>[2x]GSTKPFGVNRGLDLDKILHCYQMNDDLFMFVTWKGCSSIDAVHINDIKEAYPLQIIKYFESL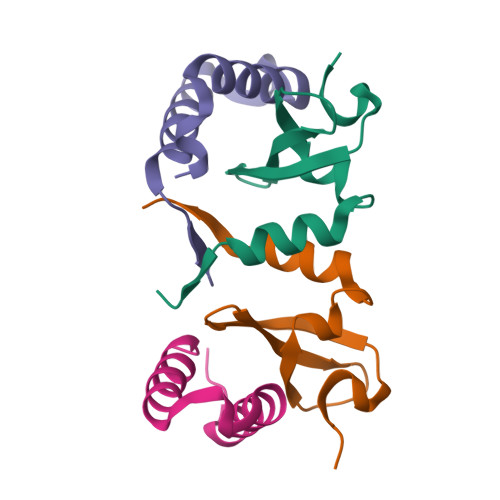RIIVPKGSGSGSGSGS;>[2x]MEKLDKIRMSQKLSCWQHILTTLGTSSKTEQEWNTFFKGFLESWRKPYCIQTSCDPSIPL> MMFGRFTERAQKVLALAQEEALRLGHNNIGTEHILLGLVREGEGIAAKALQALGLGSEKIQKEVESLIGRGQEMSQTIHYTPRAKKVIELSMDEARKLGHSYVGTEHILLGLIREGEGVAARVLNNLGVSLNKARQQVLQLLGSNETGSSAAGTNSNANTPTLD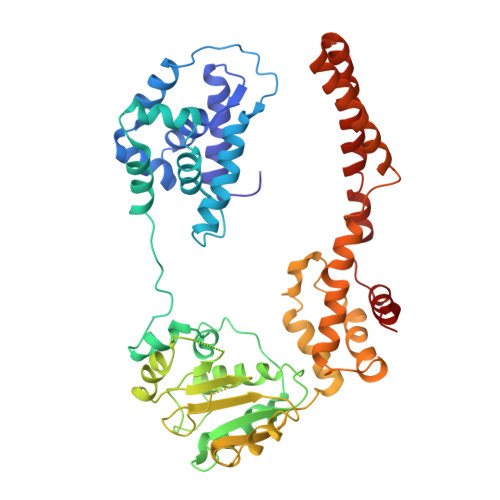SLARDLTAIAKEDSLDPVIGRSKEIQRVIEVLSRRTKNNPVLIGEPGVGKTAIAEGLAQQIINNEVPEILRDKRVMTLDMGTKYRGEFEDRLKKVMDEIRQAGNIILFIDAAIDASNILKPSLARGELQCIGATTLDEYRKYIEKDAALERRFQPIQVDQPSVDESIQILQGLRDRYEAHHRVSITDDAIEAAVKLSDRYISDRFLPDKAIDLIDEAGSKVRLRSFTTPPNLKELEQKLDEVRKEKDAAVQSQEFEKAASLRDTEQRLREQVEDTKKSWKEKQGQENSEVTVDDIAMVVSSWTG> MTLSHLVDVVRRAHPDVDLEGAGVHSGQFHDVLIARDRVFRFPKTAGAAAELPGRVAVLTAVDAVELGVGVPVPLSEVRDGGPHGFLVLSRLHGTPLERGDATSPEVIDVVAAEFARVLRAMAGADVEKLRLVLPVADAGRWRGFAGRVRATLFPLMSEDGRARAERELAAAVAMDHVATGLVHGDLGGENVLWQQVEELPRLTGIVDWDEAKVGDPAEDLAAVGASYGPELVERVVALLGAGDLWPRIRAYQGTFALQQALAGAEDGDDEELEDGLTAYRKLAAALEHHHHH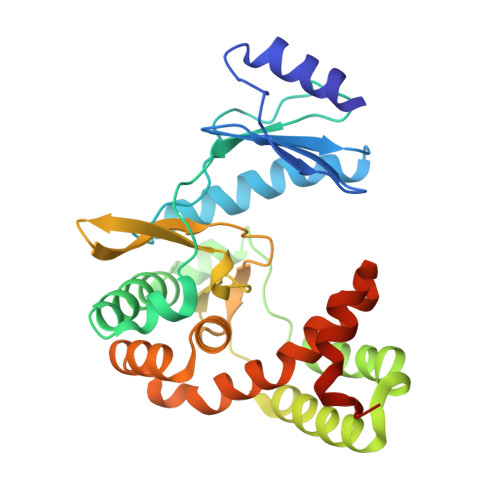H> MGSSHHHHHHSSENLYFQGAMKLIIAGKNNIAVDVTKWIIKTISDIELYSVCNENDHGNDSFQLSFKKFCIQFNIPIISLEDAYHLEDAIFLSLEFDKIIHPSKFTHNRIFNIHFSYLPAYKGMYTSAWPILNNEQESGVTLHKIDHGIDTGAIIDQQKFPLDIEETAKTLYLKYIKIGTEIVIKNLPALISGNYSIVEQSA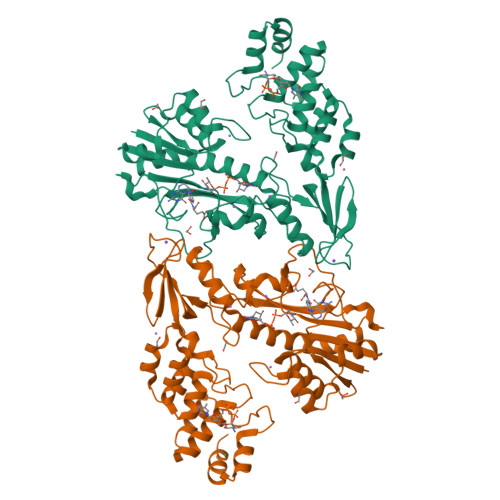IKSSYYSKKSIDYKNLMIDLNKTAHEILQQIRAFTFRDYQLPRIDDIDIFHGEILSSKSLSKPGTILEKNNYHLILSTIDYDIKLYSDNFDEILTACEDKSPEFISKLLKTENILFEKNHLGWSPIIIAAYHGNMDVIEWLVSKGVNINDRNYKGTTVAMYFKDYMLRSGNYTGLENLINLGLDLFLKDNEGLSVFDYMRKNKNIELFNFMSTFN>GKFKLVFLGEQSVGKTSLITRFMYDSFDNTYQATIGIDFLSKTMYLEDRTVRLQLWDTAGQERFRSLIPSYIRDSTVAVVVYDITNLNSFQQTSKWIDDVRTERGSDVIIMLVGNKTDLADKRQITIEEGEQRAKELSVMFIETSAKTGYNVKQLFRRVASALLEH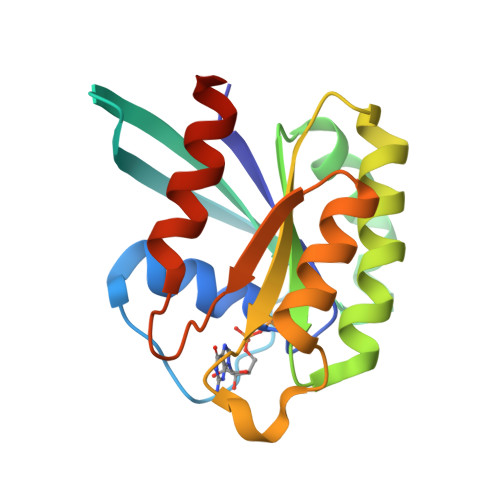HHHHH[3x]In the PT-based defense system Ssp, SspABCD confers a single-stranded PT modification of host DNA in the 5′-CPSCA-3′ motif and SspE impedes phage propagation. Notably, SspABCD coupled with SspE confers resistance to a wide array of phages through unusual mechanisms: (1) SspE is a dual-function protein that exerts both N-terminal NTPase and C-terminal DNA nicking nuclease activities to defend against phage infection, and (2) NTPase activity, including GTPase, CTPase, and UTPase activity, is stimulated exclusively by 5′-CPSCA-3′-containing DNA in vitro. Here, structural and biochemical analyses reveal that SspE is preferentially recruited to PT sites mediated by the joint action of its N-terminal domain (NTD) hydrophobic cavity and C-terminal domain (CTD) DNA binding region. PT recognition enlarges the GTP-binding pocket, thereby increasing GTP hydrolysis activity, which subsequently triggers a conformational switch of SspE from a closed to an open state.

However, the side chains of the C-terminal half, including residues 327-771, could not be resolved due to the mediocre resolution of the X-ray diffraction. The crystal structure had four molecules in the asymmetric unit of SspECTD. Each molecule exhibited an α-helical fold with only a handful of β-sheets.

>[4x]SLNTTGEPLTAFETFLPRVVMAEKIQDYQDSDAHEYMKAVQGYLDRFAVGDRLQNATRDLLVTFALAETGEKLSKRLPDQRVYMRDTFERHKDSADDRSAYLRHLRDTAAFIGNAWEPANNSPRALPGLEASAMTDTVKLCLAFLNSLKHTIAIAPLVRFYSEAVHADEGEAREKRVAEFEKAIKAITAFTVFWRATRRGTGNIDSQYRAVMAGADSLTGIGPLARQWAEPDATKPDPDVDAEALKKELAARLSDPKGKGGVPNLASFLADASALPLYKISPPLARFLLLAAYHDTIEDPDNPGLIVQGKAGVASCFTADGWEDDTHLTIEHIAPQSATSGWDAEFYSDKETVHKLGNLVLAPGAANASLSSRPWTEKKVLYAALGASTADDAKSILNSSGFTFAQTTEDLAAMSRYLPHLRALGQREDELDPAFMDQRADVLLRLAYTRLKGWLGLELSDSSSDPVVKVDDVEVENGELDESGDAGAVVGTA2-O-[(R)-{[(2S)-1,1-dihydroxypropan-2-yl]oxy}(hydroxy)phosphoryl]-beta-D-glucopyranose | C9 H19 O11 P | 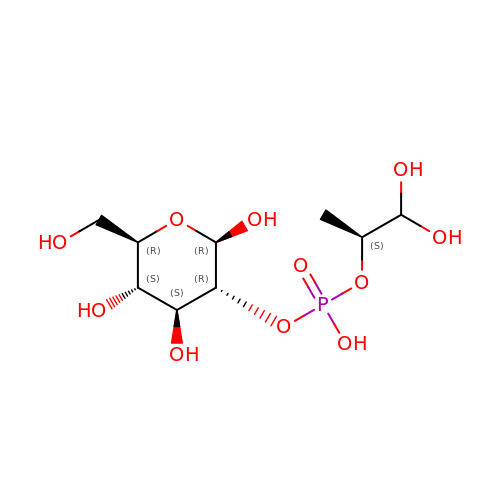SILWFZFNYLTARD-AVLLYLPDSA-N>MKIGIGSDHGGYNLKREIADFLKKRGYEVIDFGTHGNESVDYPDFGLKVAEAVKSGECDRGIVICGTGLGISIAANKVPGIRAAVCTNSYMARMSREHNDANILALGERVVGLDLALDIVDTWLKAEFQG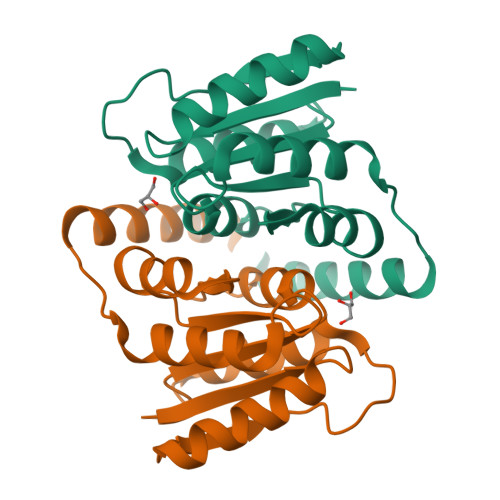GRHATRVGKIGEIEKKYSK[2x]> ETLEDS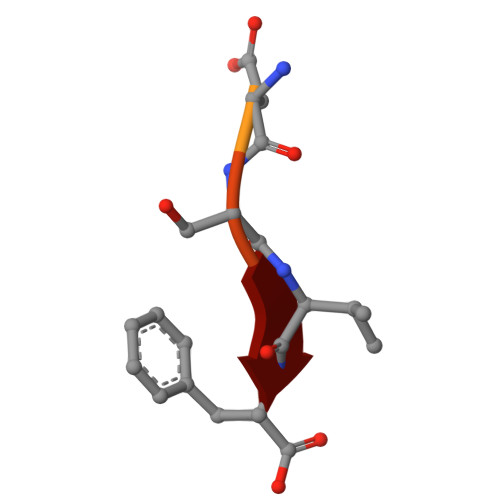VF> MVGALLLASCKQAEEPKVAEKKAPVKVILVEAQIPPKPVKPPLPPLFSDIERRTFQFFWDTTNELNGLSPDRFPSRPFASIASVGFALTAYPIGIENGWVSRNQAIDRTLTTLKFFRDAPMGPQRTGKAGYKGFYYHFLDMQQGNRYDSWVELSSVDTALLMMGVLFTQSYYDGDDPREKEIRQIADTLYKRVDWR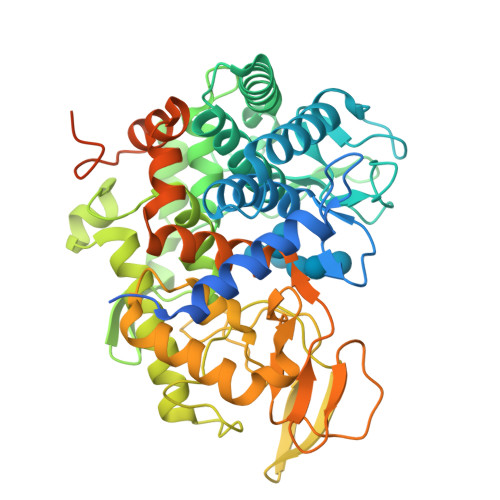WLQQRAPLISMGWFPESGFIDHDWMGYNQAMMLYILALGSPTHGVEPDAWTVWTRTYNNDWGVYQGQEYLSFGPMFGHQYSHVWIDFRDIQDQYMRERGIDYFLNSRRATLAQRDYAIDNPMKWKDYGENVWGLTAGDGPQNTSQEYRGEQRQFRHYSSRGAGLRENFDDGTIAPTAAISSIVFAPEVVIPATEEMHKRYGDFLYSSYGFLDSFNPSFNYDIPLKTGRMVPDRGWVASDYIAIDQGPILAMIANYQNEFVWNVMKKNAYIRTGLERAGFTGGWLTPDGEPQPLPKKDEQAAAARALGMAESRAAAAQAQQDPSQRQHSSQRPKPELEHHHHHH>ETLVKVKDAEDQLGARVGYIELDLNSGKILESFRPEERFPMMSTFKVLLCGAVLSRVDAGQEQLGRRIHYSQNDLVEYSPVTEKHLTDGMTVRELCSAAITMSDNTAANLLLTTIGGPKELTAFLHNMGDHVTRLDRWEPELNEAIPNDERDTTMPVAMATTLRKLLTGELLTLASRQQLIDWMEADKVAGPLLRSALPAGWFIADKSGAGERGSRGIIAALGPDGKPSRIVVIYTTGSQATMDERNRQIAEIGASLI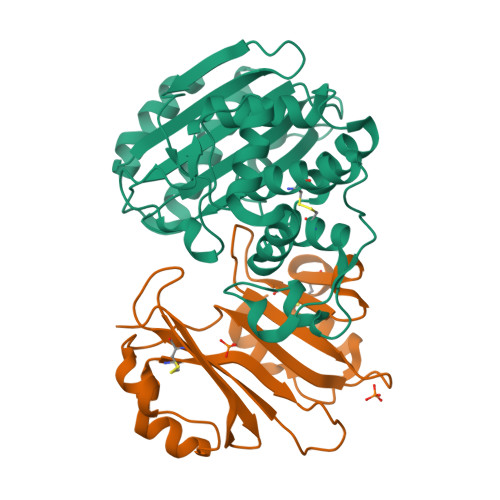KHW[2x];>SGFSAEKYEQIQFGMTFDEVWEIGGGEAACDTGGVIGDSILCFTESGDYAPYGGFSFTDEGELWSKRNEYLYKAKTPSVKLSHYNRTALGMTEAQLWAAVPKDSCVSQGESYPNWPAKTGFEEKYYCAAATGLFPPSASFHLTDGVLTYRYQRSLT[2x]>MRIVRRRPAATLLRHLALVAAALPVLAGTASAAPPTDRYAAPGLEKPASILIDRWGVPHIYAGTLYDAFYAQGFIAARDRLWQIDLWRKRGLGEMARDFGPAYVDGDRMARAVLYRGDMYREWLAYGSDAKRVAEAFVAGVNAYVALTEAQPELLPREFKQLGYKPSRWRAEDIVRIRHHGLTLNFTGEVDRATLYCQAKEQAARADWLRRELDPPITPTLPEGLDPCAVPAAALKKAYTLATAAANFPKEAWQKASADAVPVDQLYAAVDANSDTGRSLGSNNWVIAGSRTSTGRPILANDPHRAHGAPSLRYVSHLNAPGLSVIGAGEPFLPGISIGHNGTIAFGLTRFYMDQEDLYVYETDPAQPKSYRYRGRWEPMETITEKITVRGEAEPRTVTIDFTRHGPVLHADDASHRAWALRAAWLDTGMAPYFGSMDYMRATNWDQFRAAMNRWGAPGENQVYADRNGNIGWIPGGLTVIRPNWDGLFPVPGDGRYEWAGYRNMDELPWAYNPSTGHIVTANENNIPPDHPAAKLGVGYEWSDSSRARRLKSLVAAAPVSSLRDSIAWQNDTVSLPAQRTLAVMRTVGNAGAAAS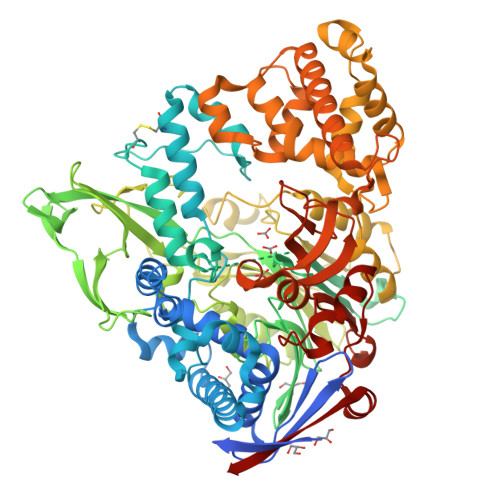LLQDPQVQRAVALLRGWDGNVRADSVPAALFEIWFSNHLRQAVVRAALPEDAAKLVGAGDAARVLAVLEQPDTWMPTARRDEVMLTSLKAAMAELERRSPSPEKLATWGTLHRAIFRHPLANIVDDATRAQYNVDAGGIGGSAFTPMNTSYRNSDYHLTAGASFRMVLDVGNWDQGRVVNTPGQSGDPGNSHYRDLAPIWAKGQTFPLVYSRKAVERAAEKRIELTPR[6x]> SAKLECPQDWLSHRDKCFHVSQVSNTW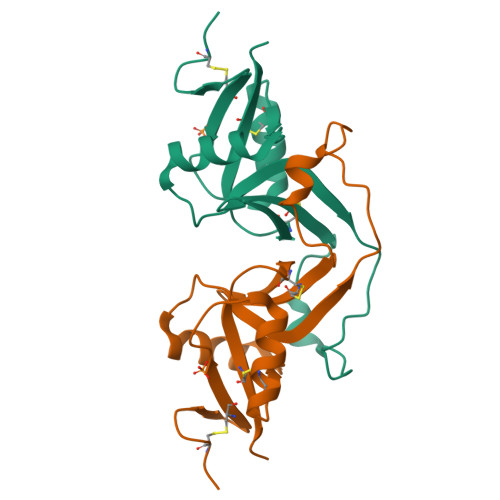EEGLVDCDGKGATLMLIQDQEELRFLLDSIKEKYNSFWIGLRYTLPDMNWKWINGSTLNSDVLKITGDTENDSCAAISGDKVTFESCNSDNRWICQKELYHETLSNYVGYGH> MGSSHHHHHHSQDPGFVFNVMCIGETGLGKSTLMDTLFNTSFESTPSPHTLPSVKLKAHTYELQESNVRLKLTICDTVGYGDQINKDDSFKAVVDYIDAQFENYLQEELKIKRSLVTCHDSRIHICLYFICPTGHGLK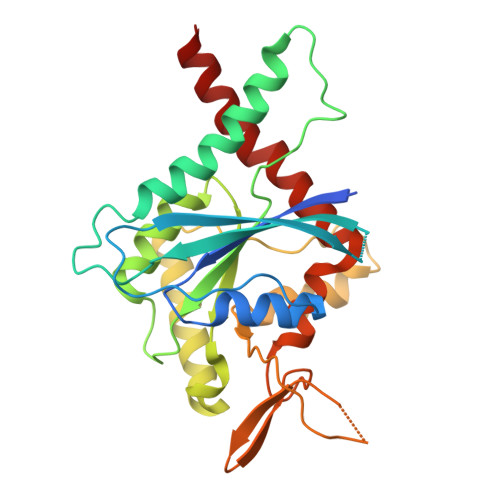SLDLVCMKKLDSKVNIIPVIAKADTISKVELQRFKAKIIQELNANGVHIYQFPTDDETVAETNTSMNSHIPFAVVGSTEFIKVGNKLIRARQYPWGTVQVENETHCDFVKLREMLIRTNMEDMREKTHTRHYELYRQKRLEQMG The interaction between NOT1 and CAF1/POP2 connects the NOT module to the catalytic module and thus is central to the assembly of the CCR4–NOT complex. Given the crucial role of this interaction, we have solved the crystal structures of the isolated CAF1-binding domain of human NOT1 (residues 1093–1317) at 2.90 Å resolution and its complex with CAF1 (i.e. CNOT7) at 2.70 Å resolution. The structures reveal that the CAF1-binding domain of NOT1 adopts an MIF4G fold; thus, this domain was termed the NOT1 MIF4G domain. CAF1 (i.e. CNOT7) and POP2 (i.e. CNOT8) are one-domain proteins that adopt an RNase D-like fold.

The crystals contain three complexes per asymmetric unit. The final structural model includes all residues of the NOT1 MIF4G domain and residues Q10–S266 and G274–E280 of CAF1 (chain B). The NOT1 MIF4G domain binds the convex surface of CAF1. The buried interface is relatively small (712 Å2) and exhibits both shape and charge complementary. The interaction is mediated primarily by residues from loops L(α6–α7) and L(α8–α9) in NOT1 and by residues from α-helices α1, α5, α6 and α7 in CAF1. Most prominently, NOT1 residue P1257 (at the N-terminus of α-helix α9) functions as a central knob; it inserts into the CAF1 surface between α-helices α5 and α6 and contacts A137, M141 (α-helix α5) and the C-beta atom of N171 (after the end of α-helix α6). The MIF4G domain of NOT1 binds CAF1 opposite to its catalytic site, leaving the catalytic residues accessible to RNA substrates. Due to the presence of 200 mM MgCl2 in the crystallization condition, we can now observe electron density for the catalytic metal ions in the human enzyme. Difference density in the active site was attributed to two hydrated magnesium ions (MgA and MgB) and a glycerol molecule from the solvent. In the structure of the NOT1-CAF1 complex, the C-terminal CAF1 fragment encompassing residues G274–E280 is visible in the electron density. This fragment includes three consecutive glutamates (E278–E280) and shields the active site of the enzyme.

>HMLEENIQEKIAFIFNNLSQSNMTQKVEELKETVKEEFMPWVSQYLVMKRVSIEPNFHSLYSNFLDTLKNPEFNKMVLNETYRNIKVLLTSDKAAANFSDRSLLKNLGHWLGMITLAKNKPILHTDLDVKSLLLEAYVKGQQELLYVVPFVAKVLESSIRSVVFRPPNPWTMAIMNVLAELHQEHDLKLNLKFEIEVLCKNLALDINELKPGNLLKDKDRLKNLDEQLS[3x];>[3x]MPAATVDHSQRICEVWACNLDEEMKKIRQVIRKYNYVAMDTEFPGVVARPIGEFRSNADYQYQLLRCNVDLLKIIQLGLTFMNEQGEYPPGTSTWQFNFKFNLTEDMYAQDSIELLTTSGIQFKKHEEEGIETQYFAELLMTSGVVLCEGVKWLSFHSGYDFGYLIKILTNSNLPEEELDFFEILRLFFPVIYDVKYLMKSCKNLKGGLQEVAEQLELERIGPQHQAGSDSLLTGMAFFKMREMFFEDHIDDAKYCGHLYGLGSGSSYVQNGTGNAYEEEANKQS> MNPKAVKRENRYANLIPMQEIKSVEQQLYPFDIYNSLRQEAPIRYDESRNCWDVFDYETVKYILKNPSLFSSKRAMEERQESILMMDPPKHTKLRNLVNKAFTPRAIQHLEGHIEEIADYLLDEVSSKEKFDIVEDFAGPLPIIVIAELLGVPIQDRALFKKYSDDLVSGAENNSDEAFAKMMQKRNEGVIFLQGYFKEIIAERQQNKQEDLISLLLEAEIDGEHLTEEEVLGFCILLLVAGNETTTNLITNGVRYMTEDVDVQNEVRRDISLVP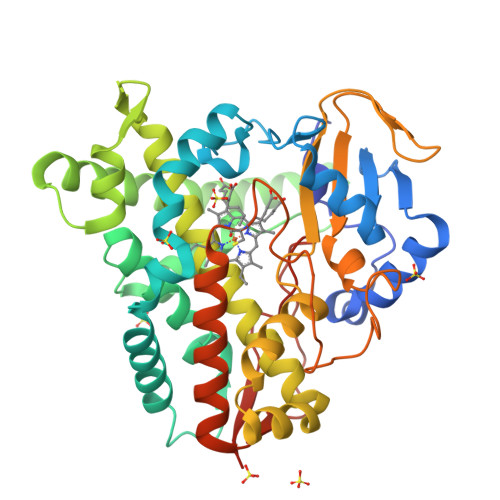NLVEETLRYYPPIQAIGRIAAEDVELGECKIKRGQQVISWAASANRDSAKFEWPDTFVVHRKTNPHVSFGFGIHFCLGAPLARMEGKIAFTKLLEKGGFSKVQNQSLKPIDSPFVFGVKKYEIAFNNAHHHHHH Anchoring of these surface proteins to the cell wall peptidoglycan requires transpeptidase enzymes called sortases, a product of an srt (surface protein sorting) gene. The membrane-associated sortase recognizes the LPXTG motif of the substrate protein, cleaves between the Thr and Gly, and forms an acyl-enzyme intermediate. According to the current model of sortase-mediated pilus assembly, the pilus polymerization catalyzed by a pilus-specific sortase is followed by cell wall anchoring of pilus polymers by the housekeeping sortase. To understand the molecular basis of pilin sorting and pilus anchoring within a bacterial strain, we investigated the housekeeping sortase, GBSSrtA, and a pilus-specific sortase, GBSSrtC1, from the PI-1 pathogenicity island of S. agalactiae SAG 2603 V/R. Either GBSSrtC1 or GBSSrtC2 of this GBS strain is capable of polymerizing GBS80, the pilus shaft of the GBS PI-1 pili.

The two molecules of the dimer, related by a non-crystallographic 2-fold axis, in the asymmetric unit of both the type II and III crystals of the GBSSrtC1 display the typical sortase fold made of an eight-stranded beta-barrel. The barrel core is flanked by two long N-terminal helices (H1 and H2), positioned approximately at 75° to each other and away from the dimer interface, which is formed by β6 strands and β4/β5 loops. Subtle differences, such as one single-turn α-helix in the β1/β2 loop present only in chain B of both dimers, and a four-turn and two-turn H1 helix in the type III and II structures, respectively, may explain the plasticity in the sortase structural features, the presence of multimers in the asymmetric unit and the observed multiple crystal-packing arrangements. Residues 44–55 and 44–54 in type II (A and B chains, respectively) and 44–51 and 46–53 in type III (chain A and B, respectively), which cover the putative active site from one-end to the other, form the lid region in GBSSrtC1. Analogous to the Asp58, Pro59 and Trp60 residues of the conserved DP(W/F/Y) motif in SPNSrtC1, Asp49, Pro50 and Tyr51 of GBSSrtC1 anchored the lid in its active site. In addition, the preceding leucine residue (Leu47) was observed inserted into a highly hydrophobic pocket in the active site present below the lid. Cys184 in the GBSSrtC1 monomers displayed a single conformation with its sulfhydryl pointing toward Arg193, which adopted a similar conformation in all of the monomers due to salt-bridge interactions with Asp49 of the lid DP(W/F/Y) motif. Arg193 also formed a weak hydrogen bond with the backbone carbonyl of Asn190, except in the type II chain A structure. Based on its lowest overall B value within the hexamer, ordered catalytic residues and positive density for all residues, we selected molecule X2 of GBSSrtA for comparison with the type II chain A molecule of GBSSrtC1.

>MRGSHHHHHHGSSHANINAFKEAVTKIDRVEINRRLELAYAYNASIAGAKTNGEYPALKDPYSAEQKQAGVVEYARMLEVKEQIGHVIIPRINQDIPIYAGSAEENLQRGVGHLEGTSLPVGGESTHAVLTAHRGLPTAKLFTNLDKVTVGDRFYIEHIGGKIAYQVDQIKVIAPDQLEDLYVIQGEDHVTLLTCTPYMINSHRLLVRGKRIPYVEKTVQKDSKTFRQQQ[2x]> M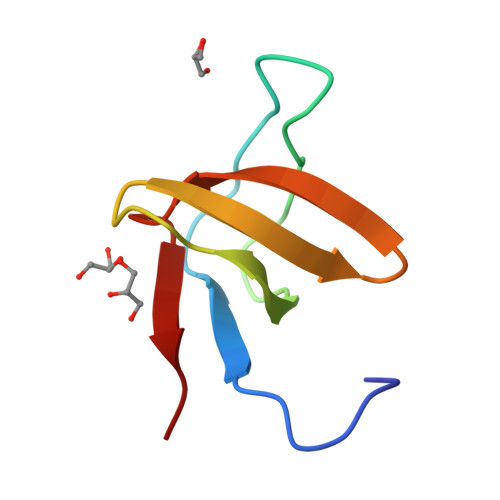DETGKELYLVLYDYQEKSPRELTVKKGDILTLLNSTNKDWWKVEVNDRQGFLPAAYLKKLD> CAGCATCGCCTGACTACA;> CGTGGACAGCGAG;> TGCTCGCTGTGGCGATGC;>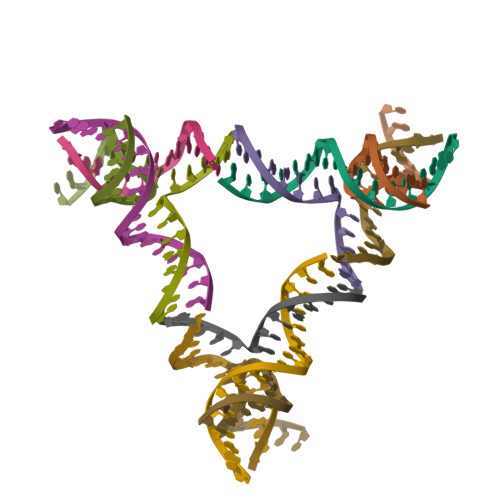 TGTAGTCACCACG>[2x]LIKHMRAEALFDFTGNSKLELNFKAGDVIFLLSRINK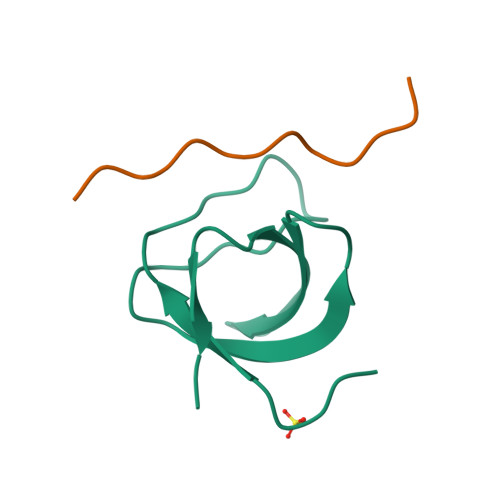DWLEGTVRGATGIFPLSFVKILK;>XKPQPAVPPRPSAD[2x]(2R)-2,5,7,8-TETRAMETHYL-2-[(4R,8R)-4,8,12-TRIMETHYLTRIDECYL]CHROMAN-6-OL | C29 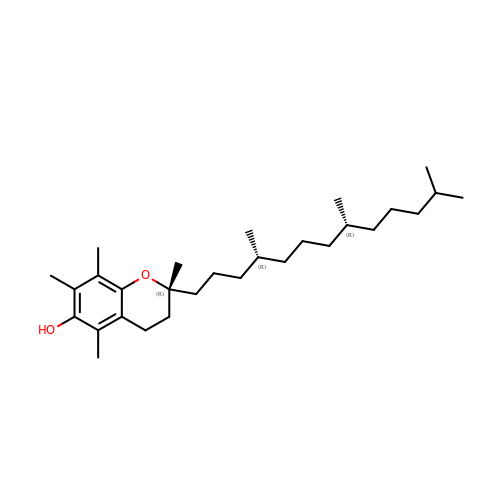H50 O2 | GVJHHUAWPYXKBD-IEOSBIPESA-N> QAFWKAVTAEFLAMLIFVLLSLGSTINWGGTEKPLPVDMVLISLCFGLSIATMVQCFGHISGGHINPAVTVAMVCTRKISIAKSVFYIAAQCLGAIIGAGILYLVTPPSVVGGLGVTMVHGNLTAGHGLLVELIITFQLVFTIFASCDSKRTDVTGSIALAIGFSVA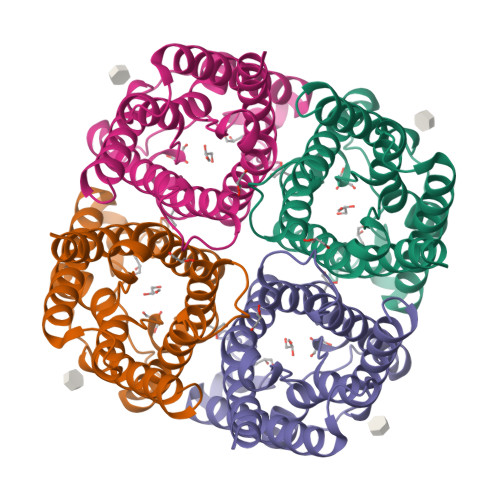IGHLFAINYTGASMNPARSFGPAVIMGNWENHWIYWVGPIIGAVLAGGLYEYVFCP>MEPTLQSILDQRSLRWIFVGGKGGVGKTTTSCSLAIQLAKVRRSVLLLSTDPAHNLSDAFSQKFGKEARLVEGFDNLYAMEIDPNGSMQDLLAGQTGDGDAGMGGVGVMQDLAYAIPGIDEAMSFAEVLKQVNSLSYETIVFDTAPTGHTLRFLQFPTVLEKALAKVSQLSGQYGSLLNGILGGSGTLPNGQTLSDVMEKLDSLRVTISEVNAQFKDERLTTFVCVCIPEFLSLYETERMIQELANYGIDTHCIVVNQLLFPKPGSDCEQCTARRRMQKKYLDQIEELYDEEFNVVKMPLLVEEVRGKERLEKFSEMLIKPFVPPEWSHPQFEK[2x];>[2x]MGRPTPLWRFLHTLLAVALGLAVIMLSPFGGTKLERDRAAAAVAGSASEREWLASLTDSYPLVKTGLGGGLFWAFATGEAILLGTRWLFLSKKKKAATAAAKVNNNNGEGDDAELDSVEQAIELALEFFPAIRQPVEYLRPKVAVAMRYVDVGMTLWRDVMLALFVLGAVAWWRAGSGSENLYFQSGSGSMSLLLVIFLLELVVQLVNTIGAKTINNLLWRFYLSIPGSPLAKDFAEQRAKQKEYLQVRHDLNATSSQDEFAKWARLQRKHDKLMDELEKKKSQLDAHRTSFSRKLTIYRWILTRGMQWFLCFWFSSQPMFWLPYGWFPYWVEWLVSFPNAPMGSVSIVVWQSACSGVLALVIEAVMAVVRYTGGTGMQKQRQPVPAAGGAPGTSKKDLGSGSLEVLFQ

The eukaryotic guided entry of tail-anchored proteins (GET) pathway mediates the biogenesis of tail-anchored (TA) membrane proteins at the endoplasmic reticulum. In the cytosol, the Get3 chaperone captures the TA protein substrate and delivers it to the Get1/Get2 membrane protein complex (GET insertase), which then inserts the substrate via a membrane-embedded hydrophilic groove. Within the membrane targeting stages of the GET pathway, the homodimeric ATPase Get3 (also called TRC40 in metazoans) adopts closed and open conformations in response to nucleotide load and interactions with other pathway components, allowing binding and release of the TA protein respectively. However, the cryo-EM structures and native mass spectrometry of hsGet1/Get2 and scGet1/Get2 show they form a 2:2 heterotetramer, which is stabilised by Get3 and interfacial lipid binding and is important for efficient TA protein insertion.

To further investigate the conformation of the GET insertase from another organism, we took advantage of the thermostability of Get1, Get2 and Get3 proteins from the thermophilic fungus Chaetomium thermophilum. A heterodimeric fusion with the flexible N-terminus of Get2 truncated (ctGet2ΔN-Get1) was recombinantly produced from S. cerevisiae and complexed with apo ctGet3 purified from Escherichia coli. We subsequently obtained single-particle cryo-EM reconstructions of both amphipol- and nanodisc-reconstituted ctGet2ΔN-Get1/Get3 at an overall resolution of 5.0 Å and 4.6 Å respectively. However, the reconstruction in amphipol additionally revealed two ~60 Å bridging helices tilted at 75o relative to the membrane normal that brace these three-TMD halves on either side (red helix). Notably, our comparison revealed the long bridging helices to be ctGet2 TMD3, which adopt the same conformation relative to ctGet1 as in hsGet1/Get2. Despite the conserved core fold, the overall morphology of the ctGet1/Get2 heterotetramer is strikingly different from the wild type human structure, as a large central membrane cavity separates the heterodimer halves. In addition, the hydrophilic groove from each heterodimer half points towards the central membrane cavity rather than to the outside, as observed in the hsGet1/Get2 heterotetramer. Finally, ctGet2 helix α3’ and the adjoining TMD3 N-terminus form the sole contact between ctGet1/Get2 heterodimers with an interface of only ~120 Å2, binding the opposing ctGet1 TMD2 instead of the ctGet3 TABD. Superimposition of ctGet3 with hsGet3 demonstrates that these changes are caused by a ~17o twist and tilt of the ctGet1 coiled-coil. Nevertheless, the structures of the wild type C. thermophilum and Δα3’ H. sapiens GET insertases represent analogous, alternative conformations of a largely conserved membrane heterotetramer, which we define as state 1.> LAAGTPALGDDRGRPWPASLAALALDGKLRTDSNATAAASTDFGNITSALPAAVLYPSSTADLVALLSAANSTPGWPYTIAFRGRGHSLMGQAFAPGGVVVNMASLGDAAA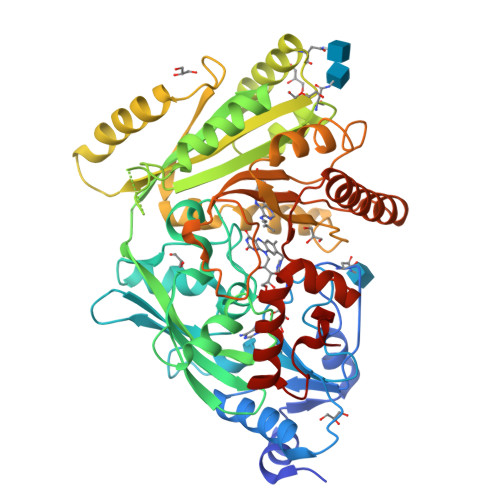PPRINVSADGRYVDAGGEQVWIDVLRASLARGVAPRSWTDYLYLTVGGTLSNAGISGQAFRHGPQISNVLEMDVITGHGEMVTCSKQLNADLFDAVLGGLGQFGVITRARIAVEPAPARARWVRLVYTDFAAFSADQERLTAPRPGGGGASFGPMSYVEGSVFVNQSLATDLANTGFFTDADVARIVALAGERNATTVYSIEATLNYDNATAAAAAVDQELASVLGTLSYVEGFAFQRDVAYAAFLDRVHGSEVALNKLGLWRVPHPWLNMFVPRSRIADFDRGVFKGILQGTDIVGPLIVYPLNKSMWDDGMSAATPSEDVFYAVSLLFSSVAPNDLARLQEQNRRILRFCDLAGIQYKTYLARHTDRSDWVRHFGAAKWNRFVEMKNKYDPKRLLSPGQDIFN>[4x]AVMAHAEGPALHPHEKLNNWGKWGDDDQRGAANYITPERIVAAARLIQT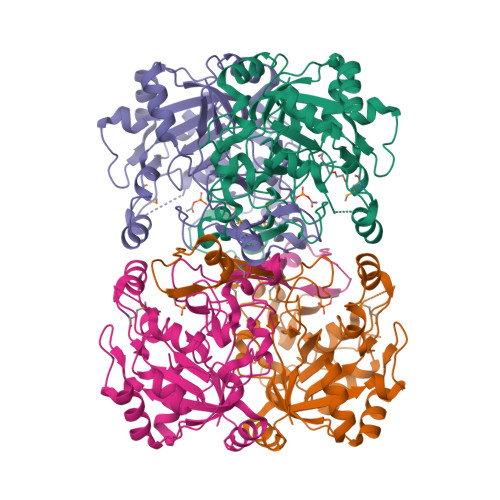GKTFSLAIPIDSNGPVFPPRLPPHHTMEITGADYVADPGASPFGKSPIRFADDYIYMPLQGSTQWDALSHGWYGESLYNGVPEAAIRSSGAGGATKLGIENVKTSFLGRGVLVDIVRFKGGSLPEGYTITRADLEGALAKQKSKLLPGDILVIRTGLVESWYDLDPVGRASFFLNPMTGIGSDTVPWIHEQRLAGVAADNIALERVPHERAPELALPVHGNLLRDLGVYIGEIWWLEELAKDCAQDGRYEFFLAAQPLYIPGAVGSPLNPIAVK>[2x]MVVIANAHNELIHDAVLDYYGKRLATCSSDKTIKIFEVEGETHKLIDTLTGHEGPVWRVDWAHPKFGTILASCSYDGKVLIWKEENGRWSQIAVHAVHSASVNSVQWAPHEYGPLLLVASSDGKVSVVEFKENGTTSPIIIDAHAIGVNSASWAPATIEEDGEHNGTKESRKFVTGGADNLVKIWKYNSDAQTYVLESTLEGHSDWVRDVAWSPTVLLRSYLASVSQDRTCIIWTQDNEQGPWKKTLLKEEKFPDVLWRASWSLSGNVLA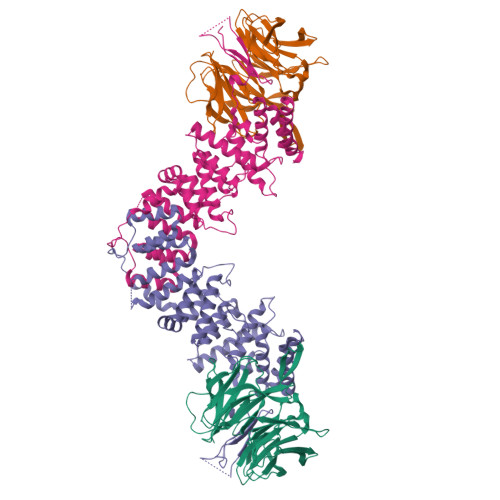LSGGDNKVTLWKENLEGKWEPAGEVHQ;>[2x]GPGSDNEALLRRQFPIFHWSAANKVVYAVPPIPDQSQYMISSSIVQEIKVTPIDQIIKPNDMLKSFPGPLGSAKLKKKDLTKWMETTIKSISENESSTDMTIWQLLEMKLNDKVNWKNISKLLYNSDELLMYLSQPFPNGDMIPNAYRLDINCQMRVLAFLQTGNHDEALRLALSKRDYAIALLVGSLMGKDRWSEVIQKYLYEGFTAGPNDQKELAHFLLLIFQVFVGNSKMAIKSFYTNNETSQWASENWKSIVAAVLINIPENNEDPLLIPPVVLEFLIEFGIFLTKKGLTAAASTLFIIGNVPLSNEPVMADSDVIFESIGNMNTFESILWDEIYEYIFSYDPKFKGFSSILPQKIYHASLLQEQGLNSLGTKYTDYLSSSVRKLPKKDILTINLTRELSEVASRLSESNTGWLAKPKLSSVWGQLDKSFNKYIGGD> MSTLQRRRVNRADSGDTSSIHSSANNTKGDKIANIAVDGDDDNGTNKKIAYDPEESKLRDNINIPTLTLMEEVLLMGLRDREGYLSFWNDSIS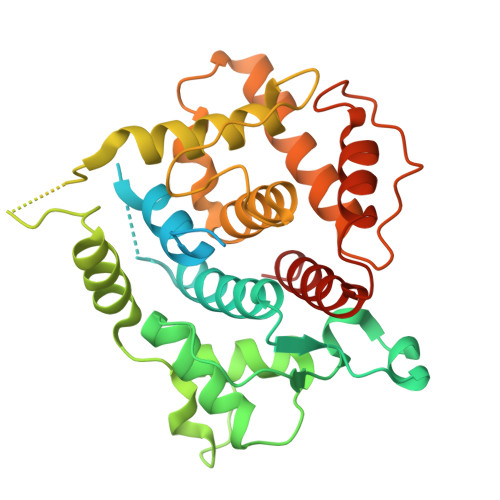YALRGCIIIELALRGKIRILDDSARKRFDLSERLIEVIDSSKTGEVLLDETLQLMKNDEPLSISNWIDLLSGETWNLLKINYQLKQVRERLAKGLVDKGVLRTEMKNFFLFDMATHPIADASCKEAIKRRVLSVLVSRNMELSYNEYFPETTSFKIIRTLALICGSYGANVLENVLTTLEYEKRDKAISRAEEIMAQFSQYPFDLEKETELGVSVNLNKEVKEEIENNPGHDLQLEVIAGVFEVFSRMDMLL The protein Roquin (encoded by Rc3h1), known to bind target mRNAs and promote their decay, has been found to be crucial in the maintenance of peripheral immune tolerance. Roquin is a ubiquitously expressed RING-E3 ubiquitin ligase family member containing a highly conserved ROQ domain required for RNA binding and localization to stress granules and a CCCH zinc finger motif. Roquin binds a stem-loop structure termed the constitutive decay element (CDE) within the 3′-UTR of Tnf mRNA and recruits the Ccr4-Caf1-Not deadenylation machinery leading to mRNA decay. mRNA degradation can also be mediated by Roquin’s recruitment of Rck/Edc4/Dcp1a decapping complexes and is thought to occur independently of miRNA activity. Our work identifies a role of the immune modulator Roquin in regulating mammalian miRNA homeostasis by promoting mature miR-146a degradation.

To gain insight into the molecular details of the interaction of Roquin with RNA, we determined the crystal structures of the ROQ domain (residues 177–326, to 2.2 Å) and a larger construct containing the RING, ROQ and zinc-finger domains (residues 1–484, to 2.75 Å) that incorporated the ‘san’ mutation M199R. There were two copies of the ROQ domain in the asymmetric unit of the first structure, with a dimer interface of 759 Å2. In Roquin, the 150-residue ROQ domain is inserted between helices 2 and 3 of the HEPN domain (beige) and is mostly α-helical. The domain boundaries differed slightly from those suggested by earlier sequence analyses. It has seven α-helices interrupted by a short β-strand between helices 2 and 3 and a β-hairpin between helices 4 and 5 (α1-α2-β1-α3-α4-α2-α3-α5-α6-α7). There are no other examples of the overall fold of the ROQ domain in the Protein Data Bank, and therefore this can be considered a new protein fold. The ROQ domain can be subdivided into an N-terminal winged helix–turn–helix (α2 to β3), followed by a C-terminal helix–turn–helix (lacking the ‘wing’ of the first, α5 to α7). These were preceded by an extra helix (α1) that appears to stabilize the relative orientation of the two sub-domains. A comparison of our Roquin1–484 structure with that of the wild-type ROQ domain demonstrated that the M199R mutation induces only a minor conformational perturbation but one that is likely to interfere with binding to either an RNA or a protein ligand. Although M199 and R199 occupied a similar spatial position, the presence of the mutation (located at the N terminus of α2) resulted in distortion of the C terminus of nearby α3 and the loop that follows it. In particular, E231 and R233 are shifted significantly and F234 flips out from its position between α2 and α3 to become completely solvent exposed.

>[2x]MLVEEEGRIRAMRAARSLGERTVTELILQHQNPQQLSSNLWAAVRARGCQFLGPAMQEEALKLVLLALEDGSALSRKVLVLFVVQRLEPRFPQASKTSIGHVVQLLYRASCFKVTKRDEDSSLMQLKEEFRTYEALRREHDSQIVQIAMEAGLRIAPDQWSSLLYGDQSHKSHMQSIIDKLQTPASFAQSVQELTIALQRTKHHHHHH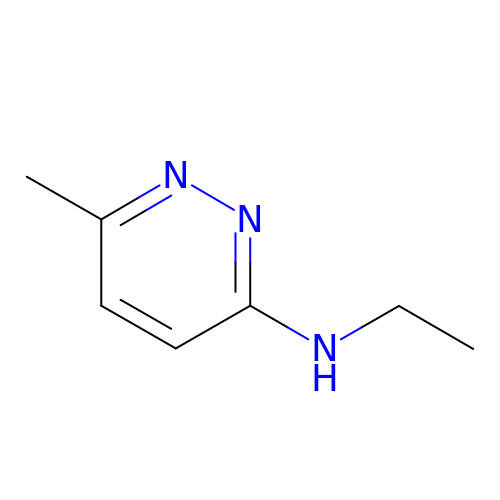N-ethyl-6-methylpyridazin-3-amine | C7 H11 N3 | RNOJUWVVUNEZSV-UHFFFAOYSA-N>[2x]MKESLKDRIRLWKRLYVNAFENALNAIPNVKGVLLAYNTNIDAIKYL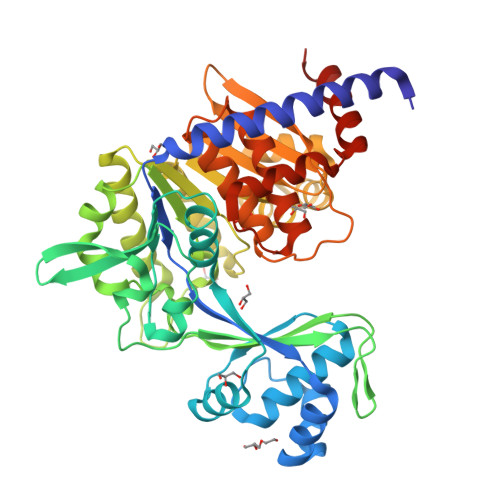DADDLEKRVTEKGKEKVFEIIENPPEKISSIEELLGGILRSIKLGKAMEWFVESEEVRRYLREWGWDELRIGGQAGIMANLLGGVYRIPTIVHVPQNPKLQAELFVDGPIYVPVFEGNKLKLVHPKDAIAEEEELIHYIYEFPRGFQVFDVQAPRENRFIANADDYNARVYMRREFREGFEEITRNVELAIISGLQVLKEYYPDGTTYKDVLDRVESHLNILNRYNVKSHFEFAYTANRRVREALVELLPKFTSVGLNEVELASIMEIIGDEELAKEVLEGHIFSVIDAMNVLMDETGIERIHFHTYGYYLALTQGGGRQLAFVPTKIVASPKSTVGIGDTISSSAFVSEFGGGGGVRDALLFASLAAAAKAMKGNLERIEQIRDALSVPTNERAIVLEEELEKEFTEFENGLIDMV> GPQTQPVPRFDETSNASGGPIKIIDPEKVSKEPDQLIEGFEWTTLDLTNETELQELWDLLTYHYVEDDNAMFRFRYSQSFLHWALMSPGWRKEWHVGVRATKSKKLV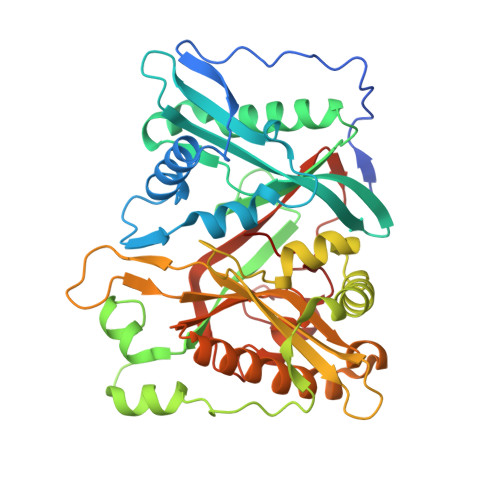ASICGVPTEIRVRDQKLKVTEINFLCIHKKLRSKRLTPVLIKEITRRCYLNGIYQAIYTAGVVLPTPVSSCRYYHRPLDWLKLYEVGFSPLPHGSTKARQITKNHLPSTTSTPGLRPMEIKDIDAVHDLLERYLKRFDMNQAFTKEEIEHWLVHKDGAGKEQVVWSYVVEDPETHKITDFFSFYNLPSTVIQHPKHKEVRAAYLYYYATETAFTEDLKALKERLLLLMNDALIQAKKAHFDVFNALTLHDNPLFLEQLKFGAGDGQLHFYLYNYRTAPIPGGVNEKNLPDEKKMGGVGVVML> MKEYTLDKAHTDVCFKIK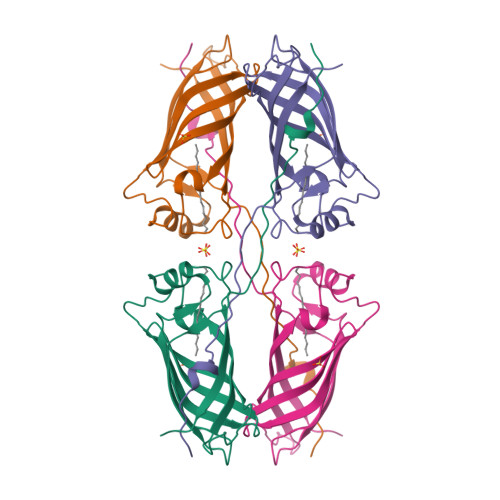HLQISNVKGNFKDYSAVIDFDPASAEFKKLDVTIKIASVNTENQTRDNHLQQDDFFKAKKYPDMTFTMKKYEKIDNEKGKMTGTLTIAGVSKDIVLDAEIGGVAKGKDGKEKIGFSLNGKIKRSDFKFATSTSTITLSDDINLNIEVEANEKEGGSHHHHHH>MAHHHHHHKKPINVAIFGSTGSIGTNALNIIRECNKIENVFNVKALYVNKSVNELYEQAREFLPEYLCIHDKSVYEELKELVKNIKDYKPIILCGDEGMKEICSSNSIDKIVIGIDSFQGLYSTMYAIMNNKIVALANKESIVSAGFFLKKLLNIHKNAKIIPVDSEHSAIFQCLDNNKVLKTKCLQDNFSKINNINKIFLCSSGGPFQNLTMDELKNVTSENALKHPKWKMGKKITIDSATMMNKGLEVIETHFLFDVDYNDIEVIVHKECIIHSCVEFIDKSVISQMYYPDMQIPILYSLTWPDRIKTNLKPLDLAQVSTLTFHKPSLEHFPCIKLAYQAGIKGNFYPTVLNASNEIANNLFLNNKIKYFDISSIISQVLESFNSQKVSENS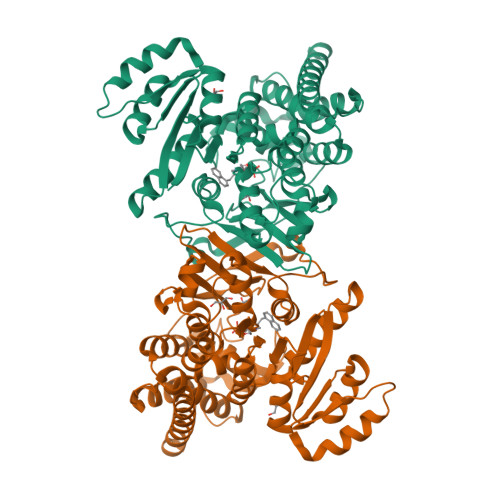EDLMKQILQIHSWAKDKATDIYNKHNSS[2x]> PQGPEIRRAADNLEAAIKGKPLTDVWFAFPQLKTYQSQLIGQHVTHVETRGKALLTHFSNDLTLYSHNQLYGVWRVVDTGEEPQTTRVLRVKLQTADKTILLYSASDIEMLRPEQLTTHPFLQRVGPDVLDPNLTPEVVKERLLSPRFRNRQFA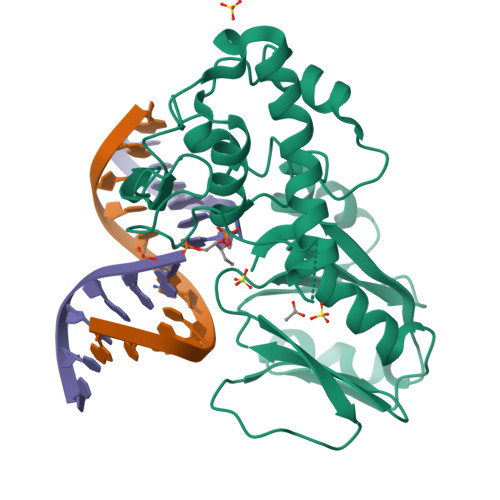GLLLDQAFLAGLGNYLRVEILWQVGLTGNHKAKDLNAAQLDALAHALLEIPRFSYATRGQVDENKHHGALFRFKVFHRDGEPCERCGSIIEKTTLSSRPFYWCPGCQH> MDGGMWLMQQINGQVARMKSLGMQLEAADIYNPNGSSLKDAVVMFDGGCTGVLVSNQGLLLTNHHCGYDQIQKHSSVQHNYLKDGFWSYSLAEELVNPGLEVEIVDEITDVTAAVKKELERIKKPSGLEFLSPRYLSSLAPEIVGKKAASRPGYRYEIKAFYGGNRYYMFTKKVFRDVRLVAAPPSSIGKFGSDTDNWAWPRHTGDFSIFRLYADKNGNPAEYSKDNVPYRPKRWVKVNAQGVKEGDFALIMGYPGTTYKFFTADEVTEWSEIDNNIRIEMRGILQDVMLREMLADPKINIMYAAKYASSQNGYKRAQGANWAIRRRSLREIKLAQQQEVLAWAKQKGIATTEEAVRAISKAIEGRQDLRMRQRYLLEGILMGIEMSNAPAADSDIADHWDDPARREAGLQSIRKQFEAFFNKDYSPEVEKDQLAIALLTRYAERIPAEKQPISIREGIAEYGSAKAYVEMIFDKSIYASRERFEEFMKNPDRDRLLRDPMSRFAASVAYEHQKLAKEVAAFDAPLAAAQRSYVASVLDMKGQPNLAPDANLTLRFTYGEIKGYQPRDVVTYGAKSTLEGVMEKEDPNNWEYVVDPKLKALYEAKNYGRYANSDGSMPVNFCATTHTTGGNAGSPVMNARGELIGLNFDRNWEGVGGDIEYLPNYQRSIILDIRYLLFIIDKFAGCQRLIDEIQPQFHHHH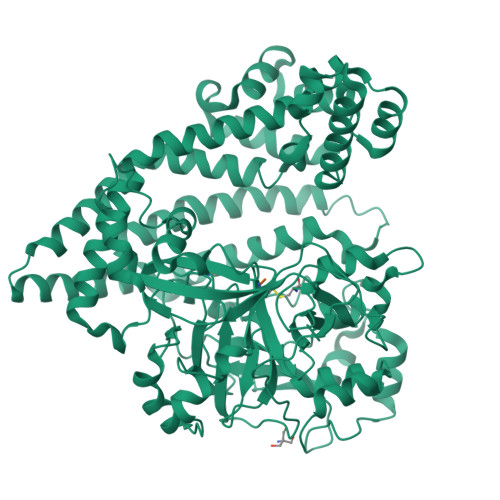HH;> LDV> AISHLNPSISKGKVHYRVPNPYIPVLLLQAVPGLGKRGELKQV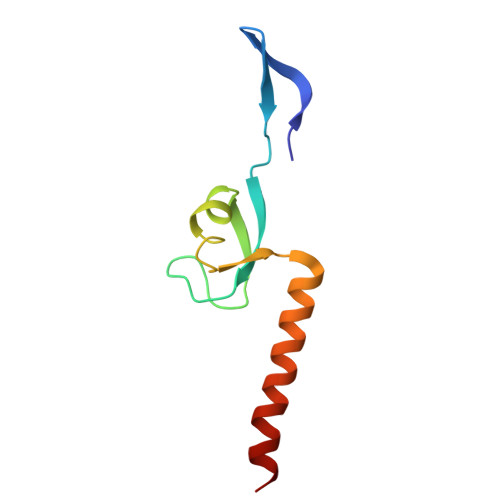RRGTLRLFLAPKGLAVVASWQNIDAFYLAEKEEEERRRRAQAGR>[2x]MRGSHHHHHHMSDEEHTFETADAGSSATYPMQCSALRKNGFVVIKSRPCKIVDMSTSKTGKHGHAKVHLVAIDIFTGKKLEDLSPST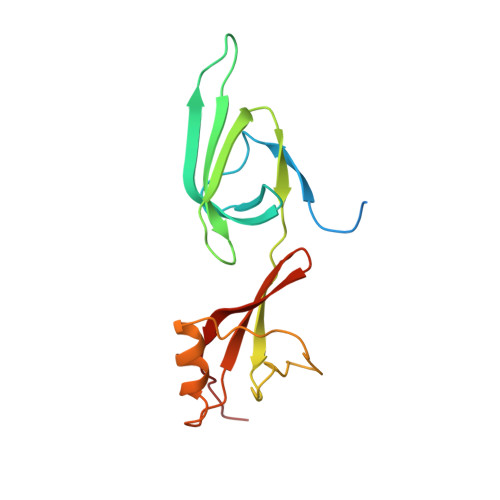HNMEVPVVKRNEYQLLDIDDGFLSLMNMDGDTKDDVKAPEGELGDSLQTAFDEGKDLMVTIISAMGEEAAISFKEAARTD>[4x]SMAVDADSANYRIEHDTMGEVRVPAKAL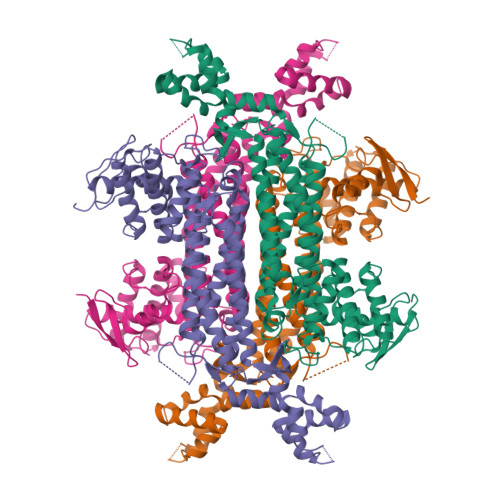WRAQTQRAVENFPISGRGLERTQIRALGLLKGACAQVNSDLGLLAPEKADAIIAAAAEIADGQHDDQFPIDVFQTGSGTSSNMNTNEVIASIAAKGGVTLHPNDDVNMSQSSNDTFPTATHIAATEAAVAHLIPALQQLHDALAAKALDWHTVVKSGRTHLMDAVPVTLGQEFSGYARQIEAGIERVRACLPRLGELAIGGTAVGTGLNAPDDFGVRVVAVLVAQTGLSELRTAANSFEAQAARDGLVEASGALRTIAVSLTKIANDIRWMGSGPLTGLAEIQLPDLQPGSSIMPGKVNPVLPEAVTQVAAQVIGNDAAIAWGGANGAFELNVYIPMMARNILESFKLLTNVSRLFAQRCIAGLTANVEHLRRLAESSPSIVTPLNSAIGYEEAAAVAKQALKERKTIRQTVIDRGLIGDRLSIEDLDRRLDVLAMAKAEQLDSDRL>ETGGTNPICKGCLSCSKDNGCLRCQPKLFFYLRREGMRQYGECLQSCPPGYYGVRGPDMNRCSRCRIENCDSCFSRDFCIKCKSGFYSHKGQCFEECPEGFAPLDDTMVCVDGTKHHHHHH[2x]

Rspo (R-spondin, also roof plate-specific spondin) proteins are evolutionarily conserved from fish to humans and have well-documented roles in a broad range of developmental and physiological processes resulting from enhancement of canonical and non-canonical Wnt signalling. ZNRF3/RNF43 specifically targets these Wnt receptors for ubiquitination and turnover, hence reducing Wnt signalling responses. Direct extracellular interaction with Rspo proteins inhibits ZNRF3/RNF43 activity. Here we report a molecular level analysis of the ZNRF3/RNF43 ectodomain structure and its interactions with Rspo proteins.

Sequence analyses suggest a putative domain structure for the Rspo proteins comprising two furin-like cysteine-rich regions (Fu domains) plus a thrombospondin type 1 repeat domain3. We therefore engineered constructs to express the region spanning the two Fu domains of Rspo2 proteins from several species. In the crystal structure of the isolated RspoFu1–Fu2 protein the two Fu domains arrange sequentially to form a ladder-like structure of β-hairpins. Each Fu domain comprises three β-hairpins rigidified by four disulphide bridges, similar to the cysteine-rich regions found in members of the epidermal growth factor receptor family. The connection between the Fu domains shows considerable rotational freedom, allowing a 50°–60° variation in the relative interdomain orientation. The N terminal of the two domains, Fu1, is distinguished by the extension of the second β-hairpin. This prominent loop presents a solvent exposed methionine (M68) at its tip, which we term the ‘Met-finger’.> AQNITARIGEPLVLKCKGAPKKPPQRLEWKLNTGRTEAWKVLSPQGGGPWDSVARVLPNGSLFLPAVGIQDEGIFRCQAMNRNGKETKSNYRVRVYQIPGKPEIVDSASELTAGVPNKVGTCVSEGSYPAGTLSWHLDGKPLVPNEKGVSVKEQTRRHPETGLFTLQSELMVTPARGGDPRPTFSCSFS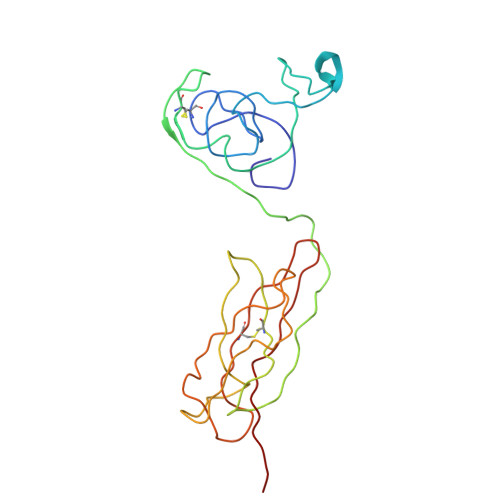PGLPRHRALRTAPIQPRVWEPV>LIIKGI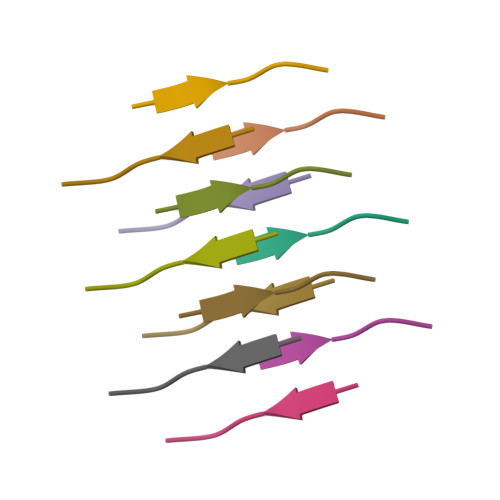[2x]> MQGTLSVWLAKRGLVHRSLGFDYQGIETLQIKPEDWHSIAVILYVYGYNYLRSQCAYDVAPGGLLASVYHLTRIEYGVNQAEEVCIKVFTHRSNPRIPSVFWVWKSTDFQERESYDMLGITYD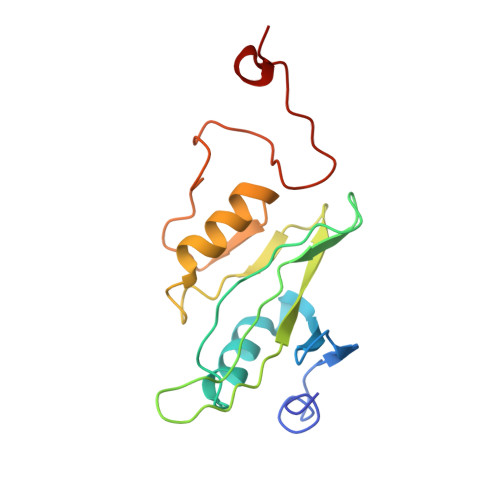SHPRLKRILMPESWIGWPLRKDYIAPNFYEIQDAY> MEDVEIKPRGYQLRLVDHLTKSNGIVYLPTGSGKTFVAILVLKRFSQDFDKPI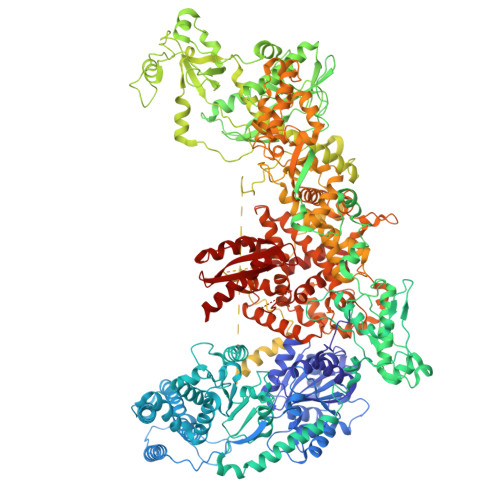ESGGKRALFMCNTVELARQQAMAVRRCTNFKVGFYVGEQGVDDWTRGMWSDEIKKNQVLVGTAQVFLDMVTQTYVALSSLSVVIIDECHHGTGHHPFREFMRLFTIANQTKLPRVVGLTGVLIKGNEITNVATKLKELEITYRGNIITVSDTKEMENVMLYATKPTEVMVSFPHQEQVLTVTRLISAEIEKFYVSLDLMNIGVQPIRRSKSLQCLRDPSKKSFVKQLFNDFLYQMKEYGIYAASIAIISLIVEFDIKRRQAETLSVKLMHRTALTLCEKIRHLLVQKLQDMTYDDDDDNVNTEEVIMNFSTPKVQRFLMSLKVSFADKDPKDICCLVFVERRYTCKCIYGLLLNYIQSTPELRNVLTPQFMVGRNNISPDFESVLERKWQKSAIQQFRDGNANLMICSSVLEEGIDVQACNHVFILDPVKTFNMYVQSKGRARTTEAKFVLFTADKEREKTIQQIYQYRKAHNDIAEYLKDRVLEKTEPELYEIKGHFQDDIDPFTNENGAVLLPNNALAILHRYCQTIPTDAFGFVIPWFHVLQEDERDRIFGVSAKGKHVISINMPVNCMLRDTIYSDPMDNVKTAKISAAFKACKVLYSLGELNERFVPKTLKERVASIADVHFEHWNKYGDSVTATVNKADKSKDRTYKTECPLEFYDALPRVGEICYAYEIFLEPQFESCEYTEHMYLNLQTPRNYAILLRNKLPRLAEMPLFSNQGKLHVRVANAPLEVIIQNSEQLELLHQFHGMVFRDILKIWHPFFVLDRRSKENSYLVVPLILGAGEQKCFDWELMTNFRRLPQSHGSNVQQREQQPAPRPEDFEGKIVTQWYANYDKPMLVTKVHRELTPLSYMEKNQQDKTYYEFTMSKYGNRIGDVVHKDKFMIEVRDLTEQLTFYVHNRGKFNAKSKAKMKVILIPELCFNFNFPGDLWLKLIFLPSILNRMYFLLHAEALRKRFNTYLNLHLLPFNGTDYMPRPLEIDYSLKRNVDPLGNVIPTEDIEEPKSLLEPMPTKSIEASVANLEITEFENPWQKYMEPVDLSRNLLSTYPVELDYYYHFSVGNVCEMNEMDFEDKEYWAKNQFHMPTGNIYGNRTPAKTNANVPALMPSKPTVRGKVKPLLILQKTVSKEHITPAEQGEFLAAITASSAADVFDMERLEILGNSFLKLSATLYLASKYSDWNEGTLTEVKSKLVSNRNLLFCLIDADIPKTLNTIQFTPRYTWLPPGISLPHNVLALWRENPEFAKIIGPHNLRDLALGDEESLVKGNCSDINYNRFVEGCRANGQSFYAGADFSSEVNFCVGLVTIPNKVIADTLEALLGVIVKNYGLQHAFKMLEYFKICRADIDKPLTQLLNLELGGKKMRANVNTTEIDGFLINHYYLEKNLGYTFKDRRYLLQALTHPSYPTNRITGSYQELEFIGNAILDFLISAYIFENNTKMNPGALTDLRSALVNNTTLACICVRHRLHFFILAENAKLSEIISKFVNFQESQGHRVTNYVRILLEEADVQPTPLDLDDELDMTELPHANKCISQEAEKGVPPKGEFNMSTNVDVPKALGDVLEALIAAVYLDCRDLQRTWEVIFNLFEPELQEFTRKVPINHIRQLVEHKHAKPVFSSPIVEGETVMVSCQFTCMEKTIKVYGFGSNKDQAKLSAAKHALQQLSKCDA>[2x]IVGGYTCGANTVPYQVSLNSGYHFCGGSLINSQWVVSAAHCYKSGIQVRLGEDNINVVEGNEQFISASKSIVHPSYNSNTLNNDIMLIKLKSAASLNSRVASISLPTSCASAGTQCLISGWGNTKSSGTSYPDVLKCLKAPILSTSSCKSAYPGQITSNMFCAGYLEGGKDSCQGDSGGPVVCSGKLQGIVSWGSGCAQKNKPGVYTKVCNYVSWIKQTIASN;>PTGNNAEICLLP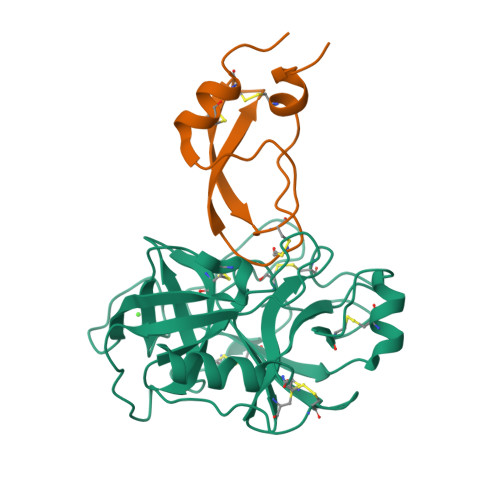LDYGPCRALLLRYYYDRYTQSCRQFLYGGCEGNANNFYTWEACDDACWRIE[2x]MYORG is a member of glycoside hydrolase (GH) family 31 (GH31) and, like the other mammalian GH31 enzyme α-glucosidase II, this enzyme is found in the lumen of the endoplasmic reticulum (ER). We were intrigued by MYORG, which is a type II transmembrane protein predicted to be comprised of a short, disordered nucleocytoplasmic N-terminal region, a single transmembrane helix, and a lumenal C-terminal catalytic region comprising a CAZy family glycoside hydrolase 31 (GH31) catalytic domain and 2 β-sheet domains. Here, we demonstrate that MYORG, enigmatically, functions not as an α-glucosidase but rather an α-galactosidase and shows marked preference for specific disaccharide substrates. Recent studies in diverse populations have shown a link between mutations in myogenesis-regulating glycosidase (MYORG) and the development of this disease.

We obtained crystals of unliganded MYORG and processed them in the P1 space group to 2.43 Å. Four copies of MYORG could be placed within the asymmetric unit (chains A to D). For chains A to C, the polypeptide backbone could be confidently traced into the electron density map, with only the first 11 amino acids (80–91) and 2 short loop regions (residues 165–171 and 270–276) proving too disordered to model. Chain C represents the most complete model of MYORG and will be used hereafter to describe the structure of MYORGGH31. Analysis of the crystal structure reveals MYORG is comprised of an antiparallel β-sandwich N-terminal domain (residues 92–287), a (β/α)8-barrel catalytic domain (residues 288–633) with an insertion between α3 and α4 (residues 393–436), and a proximal β-sheet domain (residues 634–714). Five cysteine residues are present in the structure and form 2 disulphide bonds within the N-terminal domain (C125 with C134 and C158 with C284). MYORGGH31 is predicted to have 6 N-glycosylation sites: N240, N250, N346, N372, N398, and N511. Glycosylation is observed on every polypeptide chain in the asymmetric unit, and it is possible to model N-glycans on all of the predicted N-glycosylation sites of chains B and C. The crystal structure shows that MYORG forms a 2-fold dimeric assembly, agreeing with our SEC-MALLS analysis, with the protein–protein interaction exclusively localised to the insert region. The interface covers 639 Å2 and is largely supported through a hydrophobic interaction network composed of F402, V406, L419, L422, and I429, in addition to hydrogen bonding between Y397 to E407.

>GVSLRKAERLRAELLDLKAGGFSIRNQKGEQVFRLAFRSGALDLDSCSRDGALLGCSLTADGLPLHFFIQTVRPKDTVMCYRVRWEEAAPGRAVEHAMFLGDAAAHWYGGAEMRTQHWPIRLDGQQEPQPFVTSDVYSSDAAFGGILERYWLSSRAAAIKVNDSVPFHLGWNSTERSLRLQARYHDTPYKPPAGRAAAPELSYRVCVGSDVTSIHKYMVRRYFNKPSRVPAPEAFRDPIWSTWALYGRAVDQDKVLRFAQQIRLHHFNSSHLEIDDMYTPAYGDFDFDEVKFPNASDMFRRLRDAGFRVTLWVHPFVNYNSSRFGEGVERELFVREPTGRLPALVRWWNGIGAVLDFTHPKARDWFQGHLRRLRSRYSVASFKFDAGEVSYLPRDFSTYRPLPDPSVWSRRYTEMALPFFSLAEVRVGYQSQNISCFFRLVDRDSVWGYDLGLRSLIPAVLTVSMLGYPFILPDMVGGNAVPQRTAGGDVPERELYIRWLEVAAFMPAMQFSIPPWRYDAEVVAIAQKFAALRASLVAPLLLELAGEVTDTGDPIVRPLWWIAPGDETAHRIDSQFLIGDTLLVAPVLEPGKQERDVYLPAGKWRSYKGELFDKTPVLLTDYPVDLDEIAYFTWAS[4x]>MSKILVFGHQNPDSDAIGSSYAFAYLAREAYGLDTEAVALGEPNEETAFVLDYFGVAAPRVITSAKAEGAEQ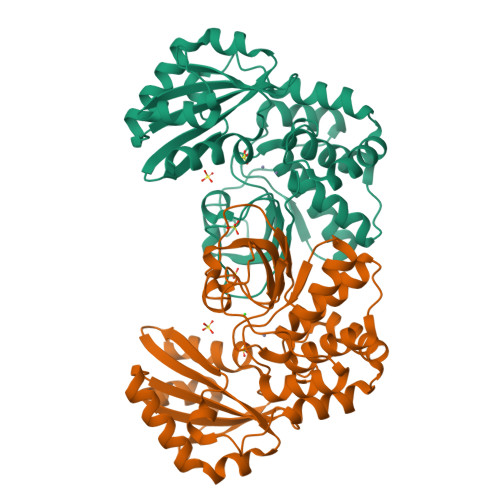VILTDHNEFQQSVADIAEVEVYGVVDHHRVANFETASPLYMRLEPVGSASSIVYRMFKEHGVAVPKEIAGLMLSGLISDTLLLKSPTTHPTDKVIAPELAELAGVNLEEYGLAMLKAGTNLASKSAEELIDIDAKTFELNGNNVRVAQVNTVDIAEVLERQAEIEAAIEKAIADNGYSDFVLMITDIINSNSEILAIGSNMDKVEAAFNFVLENNHAFLAGAVSRKKQVVPQLTESFNA[2x]>[4x]MSNCQYKIYPPLGIARVGNGPAIKPLSLSTPEVPWAHLYDTNVQYL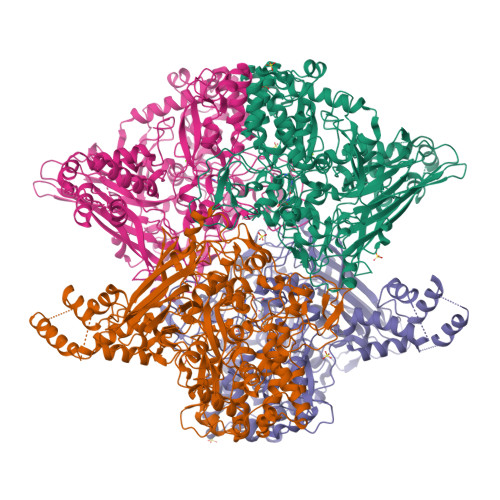VTQQELEQLLEEAFGGNVINEISQIKTKLDERKAEKFKQEEIETITGLLGLSHLVPQQQLSRSLDNLELKSTKDSDDIVQQIKGALLKVLSDHYLHAVKKQAQNFYIYKCDEQGNPVEKLKLTDGDKVTWRVEVANKKSFWYDYNNALDLSLHTQGSGNLSKNVSKHRLAPAMTAKRRNPNVITNSLRKQLVISSQGSVSSDNNTQVPLRGKFPANEPDTNNRLSDLLNLQERHNVLQGSIECDNEGVLRFYAGNGISQALSPSSLNTDFADNSNWFDDICDGRVTAVVELKNGDTFEIQDEQSSAWVATTPPDYAPQIEPIVTMYDMVSGAALKEQDLDNLTTQFSDVFPILYRLYRMQWVNQADFTDNAVNTQIRELNSELGFAQLLDNSASAKSLREGIFNQFRNPLFDQDIDVDDPGQSSNEWVSNSRIIPSKDETNIAAKPATSSLKLPFYPNDGIDYPGSPVQWFAIPPFMYQHLQNWAAGDFSVTQVEKESANTIEELGLFYSEQFKNSPNSALLCARGALDALYGGGFHPGVELTWPMRHNLIYSQNDYVSSVTPEINLLGLREFRLKQDLQGLNSPNMYQDFGHVIAVDNVTASIDPNSDAAWLWRSTPGDLTKWMGIPWQSDAASCQAVYTPEDFPIPSWWAANLPVHVLPLARYNKFKDSQSADLPEINGMTHSIAQGMSEETFEHLRLEQFSQRLDWLHTADLGFVGYAAEGGYTNGLIQMVSQWKNMAMVMARPVENPGSSGIPNVVYVAYSQADKD> GLPTRLPSGSQQFMTTEDEQSPNILPG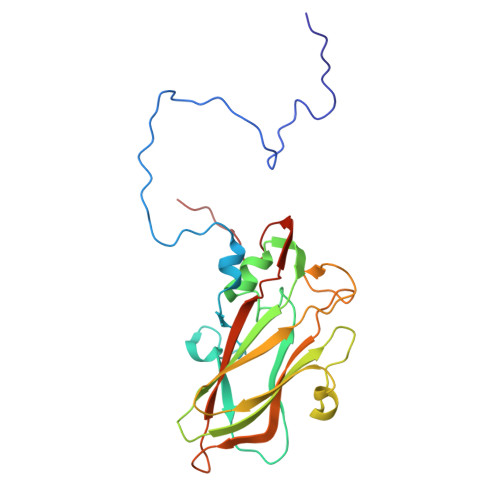FHPSKKIHIPGMITNVMHMARVDSFIPINNIQGEVGKVSMYYITVTKKTVTERILVLPLEMSNTLFATTLLGEVLNYYANWSGSITITFMCVCDAFSTGKFLVAYTPPGGKLPEDRKQAMLGVHIIWDLGLQSSCTIVVPWISSGFYRRTKADSFTHGGYVSLWYQTAFVPPVSGGTGSILATCSACPDMSVRMLRDSPMMEQKNELQ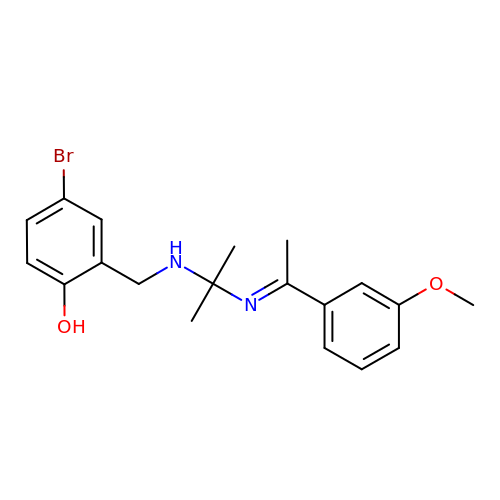4-bromanyl-2-[[2-[(E)-1-(3-methoxyphenyl)ethylideneamino]propan-2-ylamino]methyl]phenol | C19 H23 Br N2 O2 | KYCOBMQFSPNZHT-LPYMAVHISA-N> GEFTQSVSRLQSIVAGLKNAPSDQLINIFESCVRNPVENIMKILKGIGETFCQHYTQSTDEQPGSHIDFAVNRLKLAEILYYK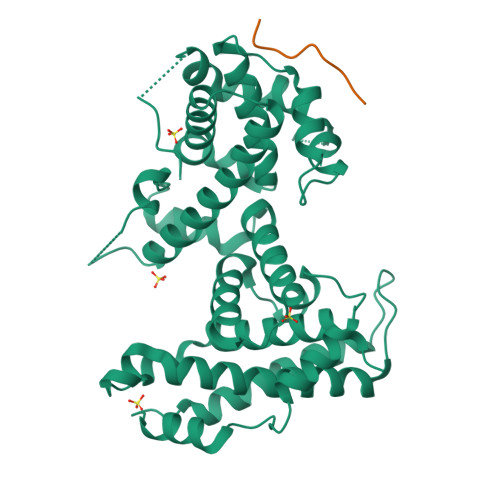ILETVMVQETRRLHGMDMSVLLEQDIFHRSLMACCLEIVLFAYSSPRTFPWIIEVLNLQPFYFYKVIEVVIRSEEGLSRDMVKHLNSIEEQILESLAWSHDSALWEALQVSANKVPTCEEVIFPNNFETGNNRPKRTGSLALFYRKVYHLASVRLRDLCLKLDVSNELRRKIWTCFEFTLVHCPDLMKDRHLDQLLLCAFYIMAKVTKEERTFQEIMKSYRNQPQANSHVYRSVLLKSIKEERGDLIKFYNTIYVGRVKSFALKYDLANQDHMMDAPPLSPFPHIKQQ;> DLYCYEQLN> IPWGGNLEEVLEELEMALLAADVGLSATEEILQEVRASGRKDLKEAVKEKLVGMLEPDERRATLRKLGFNPQKPKPVEPKGRVVLVVGVNGVGKTTTIAKLGRYYQNLGKKVMFCAGDTFRAAGGTQL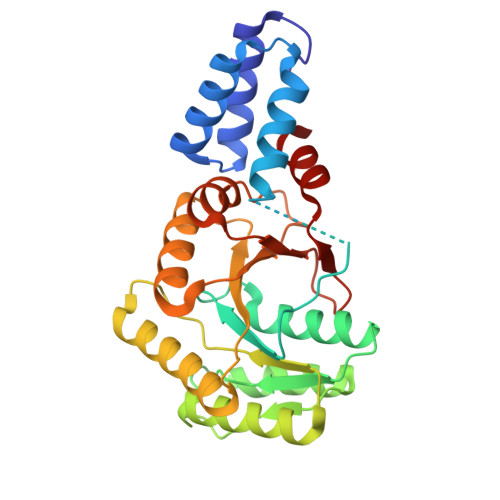SEWGKRLSIPVIQGPEGTDPAALAYDAVQAMKARGYDLLFVDTAGRLHTKHNLMEELKKVKRAIAKADPEEPKEVWLVLDAVTGQNGLEQAKKFHEAVGLTGVIVTKLDGTAKGGVLIPIVRTLKVPIKFVGVGEGPDDLQPFDPEAFVEALLED>[4x]MLARHGPRYGGSVNGHSDDSSGDAKQAAPTL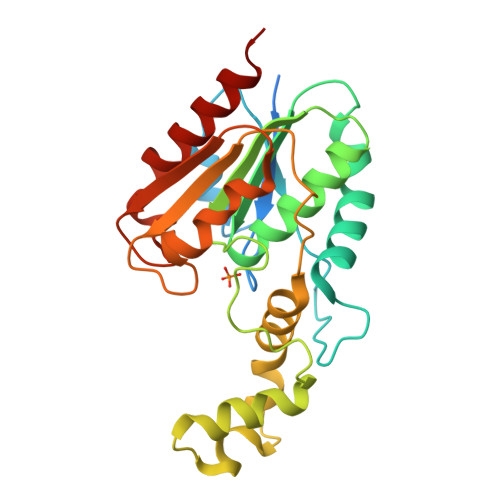YIFPHAGGTAKDYVAFSREFSADVKRIAVQYPGQHDRSGLPPLESIPTLADEIFAMMKPSARIDDPVAFFGHSMGGMLAFEVALRYQSAGHRVLAFFVSACSAPGHIRYKQLQDLSDREMLDLFTRMTGMNPDFFTDDEFFVGALPTLRAVRAIAGYSCPPETKLSCPIYAFIGDKDWIATQDDMDPWRDRTTEEFSIRVFPGDHFYLNDNLPELVSDIEDKTLQWHDRA> G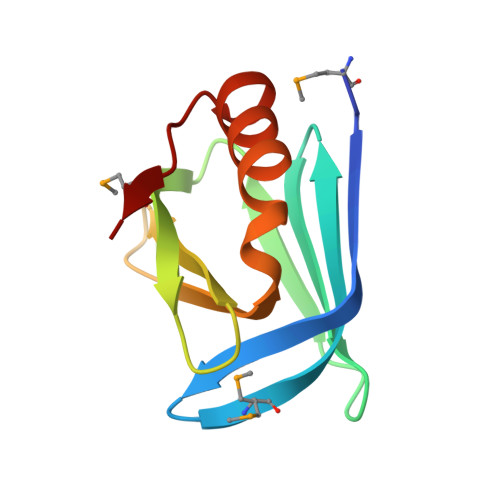HMAETLEFNDVYQEVKGSMNDGRLRLSRQGIIFKNSKTGKVDNIQAGELTEGIWRRVALGHGLKLLTKNGHVYKYDGFRESEFEKLSDFFKTHYRLELMEK>AASAQDAPEAETQAQETQGQAAARAAAADLAAGQDDEPRILEAPAPDARRVYVNDPAHAAAVTQQFVIDGEAGRVIGMIDGGFLPNPVVADDGSFIAHASTVFSRIARGERTDYVEVFDPVTLLPTADIELPDAPRFLVGTYPWMTSLTPDGKTLLFYQFSPAPAVGVVDLEGKAFKRMLDVPDCYHIFPTAPDTFFMHCRDGSLAKVAFGTEGTPEITHTEVFHPEDEFLINHPAYSQKAGRLVWPTYTGKIHQIDLSSGDAKFLPAVEALTEAERADGWRPGGWQQVAYHRALDRIYLLVDQRDEWRHKTASRFVVVLDAKTGERLAKFEMGHEIDSINVSQDEKPLLYALSTGDKTLYIHDAESGEELRSVNQLGHGPQVITTADMG[4x];>ADAPAGTDPRAKWVPQDNDIQACDYWRHCSIDGNICDCSGGSLTNCPPGTKLATASWVASCYNPTDGQSYLIAYRDCCGYNVSGRCPCLNTEGELPVYRPEFANDIIWCFGAEDDAMTYHCTISPIVGKAS[4x];>DKATIPSESPFAAAEVADGAIVVDIAKMKYETPELHVKVGDTVTWINREAMPHNVHFVAGVLGEAALKGPMMKKEQAYSLTFTEAGTYDYHCTPHPFMRGKVVVE[4x];>[4x]APQFFNIIDGSPLNFDDAMEEGRDTEAVKHFLETGENVYNEDPEILPEAEELYAGMCSGCHGHYAEGKIGPGLNDAYWTYPGNETDVGLFSTLYGGATGQMGPMWGSLTLDEMLRTMAWVRHLYTGDPKDASW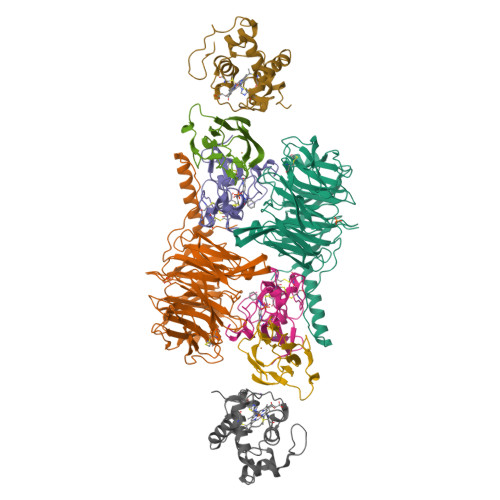LTDEQKAGFTPFQPKSSGEDQS> MSLELQEHCSLKPYNTFGIDVRARLLAHARDEADVREALALARERGLPLLVIGGGSNLLLTRDVEALVLRMASQGRRIVSDAADSVLVEAEAGEAWDPFVQWSLERGLAGLENLSLIPGTVGAAPMQNIGAYGVELKDVFDSLTALDRQDGTLREFDRQACRFGYRDSLFKQEPDRWLILRVRLRL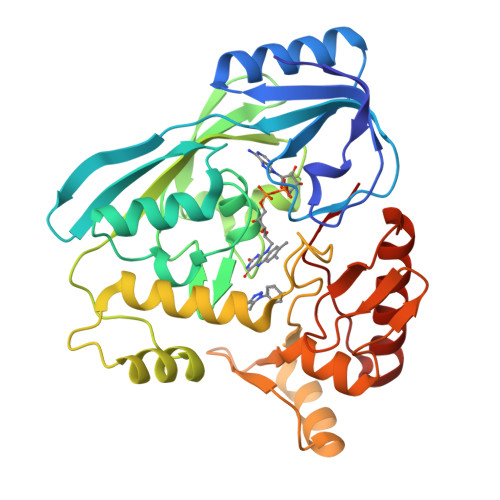TRRERLHLDYGPVRQRLEEEGIASPTARDVSRVICAIRREKLPDPAVLGNAGSFFKNPLVDATQAERLRQAFPDLVGYPQADGRLKLAAGWLIDKGGWKGFRDGPVGVHAQQALVLVNHGGATGAQVRALAERIQEDVRRRFGVELEPEPNLY>[4x]GAMTAFRIEKDTMGEVQVPADKYWAAQTERSRNNFKIGPAASMPHEIIEAFGYLKKAAAFANTDLGVLPAEKRDLIGQACDEILARKLDDQFPLVIWQTGSGTQSNMNLNEVIANRAHVINGGKLGEKSIIHPNDDVNKSQSSNDTYPTAMHIAAYKKVVEATIPAVERLQKT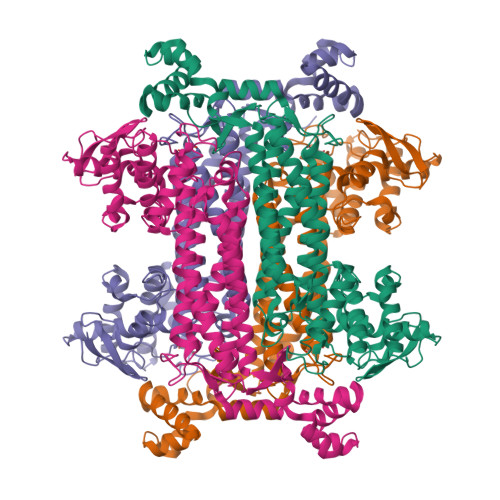LAAKAAEFKDVVKIGRTHLMDATPLTLGQEFSGYAAQLSFGLTAIKNTLPHLRQLALGGTAVGTGLNTPKGYDVKVAEYIAKFTGLPFITAENKFEALATHDAIVETHGALKQVAMSLFKIANDIRLLASGPRSGIGEILIPENEPGCSIMPGKVNPTQCEAMTMVAAQVLGNDTTISFAGSQGHFELNVFKPVMAANFLQSAQLIADVCISFDEHCATGIQPNTPRIQHLLDSSLMLVTALNTHIGYENAAKIAKTAHKNGTTLREEAINLGLVSAEDFDKWVVPADMVGSLK ClfB, an MSCRAMM (Microbial Surface Components Recognizing Adhesive Matrix Molecules) family surface protein, described as a fibrinogen-binding clumping factor, is a key determinant of S. aureus nasal colonization, but the molecular basis for ClfB-ligand recognition remains unknown. ClfB plays a key role in establishing human nasal colonization by binding to the human type I cytokeratin 10 (CK10) expressed on squamous epithelial cells. As a bifunctional MSCRAMM, ClfB also binds to fibrinogen α (Fg α), which is assumed to be significant in platelet activation and aggregation and has been shown to contribute to the pathogenesis of experimental endocarditis in rats. In this study, we solved the crystal structures of apo-ClfB and its complexes with fibrinogen α (Fg α) and cytokeratin 10 (CK10) peptides.

To this end, we synthesized a 15-amino-acid-peptide (250–264; GQSGSSGSGSNGDNN, designated as Derm15 hereafter) derived from Derm and then characterized its binding to ClfB using the SPR (Surface Plasmon Resonance) assay. In the assay, ClfB bound to the peptide with a dissociation constant of 2.37 µM. Interestingly, the results also showed that the Derm peptide interacted with ClfB with slow kinetics, further supporting the DLL model. To understand the molecular mechanism underlying this interaction, we solved the crystal structure of ClfB(208–542) bound to the peptide at 2.5 Å resolution. As expected, Derm15 interacts with ClfB in a nearly identical manner with Fg α(316–328) and CK10(499–512). The ClfBArg529 forms a hydrogen bond with ClfBAsn328 and the C-terminus of N3 forms an extra strand, which is similar as that in the ClfB-Fg α(316–328) and ClfB-CK10(499–512) complexes. While the wild type ClfB bound tightly to Derm15, the mutant proteins ClfB(197–542) S236A or W522A exhibited much lower binding affinities with the peptide in mM range. Interestingly, besides the low binding affinities, both mutant proteins exhibited rapid association and dissociation behaviors in the experiments, as compared to the slow association and scarcely any dissociation behaviors observed for the wild type protein. These results indicated that the residues ClfBS236, W522 are not only involved in the binding with ClfB, but also participate in stabilizing or “locking” the peptide in place. Further supporting this prediction, our structural studies revealed that the binding mode of the Dermokine-derived peptide to ClfB is nearly identical with that of the Fg α/CK10-derived peptide.

> MRGSHHHHHHENLYFQGSLAVAEPVVNAADAKGTNVNDKVTASDFKLEKTAFDPNQSGNTFMAANFKVTGQVKSGDYFTAKLPDSVTGNGDVDYSNSNNTMPIADIKSTNGDVVAKATYDILTKTYTFVFTDYVNDKENINGQFSLPLFTDRAKAPKSGTYDANINIADEMFDNKITYNYSSPIAGIDKPNGANISSQIIGVDTASGQNTYKQTVFVNPKQRVLGNTWVYIKGYQDKIEESSGKVSATDTKLRIFEVNDTSKLSDSYYADPNDSNLKEVTGEFKDKISYKYDNVASINFGDINKTYVVLVEGHYDNTGKNLKTQVIQENIDPATGKDYSIFGWNNENVVRYGGGSADGDSAVN;> GQSGSSGSGSNGD>[2x]MRFIHALLLAGIAHSAYASEKLTFKTDLEKLEREKAAQIGVAIVDPQGEIVAGHRMAQRFAMCSTFKFPLAALVFERIDSGTERGDRKLSYGPDMIVEWSPATERFLASGHMTVLEAAQ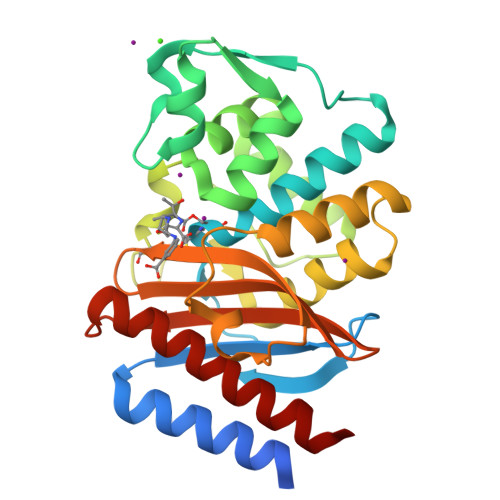AAVQLSDNGATNLLLREIGGPAAMTQYFRKIGDSVSRLDRKEPEMNDNTPGDLRDTTTPIAMARTVAKVLYGGALTSTSTHTIERWLIGNQTGDATLRAGFPKDWVVGEKTGTCANGGRNDIGFFKAQERDYAVAVYTTAPKLSAVERDELVASVGQVITQLILSTDK>SNQLVVAFKEDNTVAFKHLFLKGYSGTDEDDYSCSVYTQEDAYESIFFAINQYHQLKDITLGTLGYGENEDNRIGLKVCKQHYKKGTMFPSNETLNIDNDVELDCVQLDLQDLSKKPPDWKNSSFFRLEFYRLLQVEISFHLKGIDLQTIHSRELPDCYVFQNTIIFD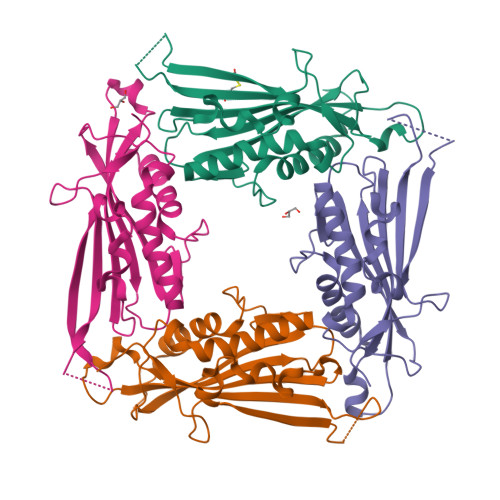NKAHSGKIKIYFDSDAKIEECKDLNIFGSTQ[8x]>[8x]MRGSHHHHHHGSMSNKIMKTSRLTAEDINGAWTIMPTPSTPDASDWRSTATVDLEETARIVEELIAAGVNGILSMGTFGECATLTWDEKRDYVSTIVETIRGRVPYFCGTTALNTREVIRQTRELIDIGANGTMLGVPMWVKMDLPTAVQFYRDVADA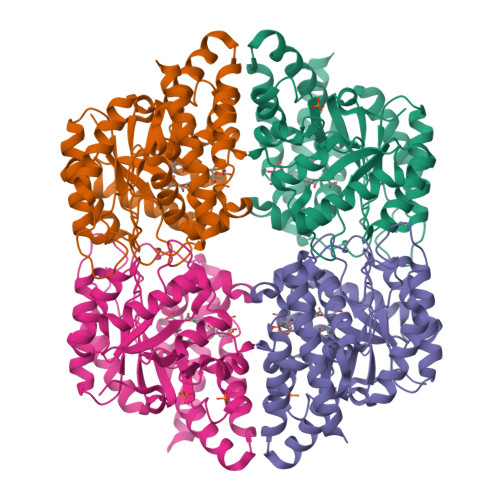VPEAAIAIYANPEAFKFDFPRPFWAEMSKIPQVVTAKYLGIGMLDLDLRLAPNIRFLPHEDDYYAAARINPERITAFWSSGAMCGPATAIMLRDEVVRAKSTGDWAKAKAISDDMRAADSTLFPRGDFSEFSKYNIGLEKARMDAAGWLKAGPCRPPYNLVPEDYLAGAQKSGKAWAALHAKYSNELK N-{3-[(2R,3R)-5-amino-3-methyl-2-(trifluoromethyl)-3,6-dihydro-2H-1,4-oxazin-3-yl]-4-fluorophenyl}-3,5-dichloropyridine-2-carboxamide 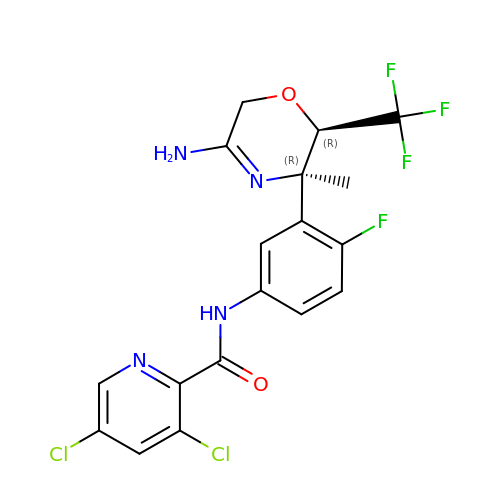| C18 H14 Cl2 F4 N4 O2 | VLILPGWCHAEKPY-IAGOWNOFSA-N>[12x]TKDNLTGDIVIIGAGAAGSLLAHYLARFSNMKIILLEAGHSHFNDPVVTDPMGFFGKYNPPNENISMSQNPSYSWQGAQEPNTGAYGNRPIIAHGMGFGGSTMINRLNLVVGGRTVFDNDWPVGWKYDDVKNYFRRVLVDINPVRDNTKASITSVALDALRIIAEQQIASGEPVDFLLNKATGNVPNVEKTTPDAVPLNLNDYEGVNSVVAFSSFYMGVNQLSDGNYIRKYAGNTYLNRNYVDENGRGIGKFSGLRVVSDAVVDRIIFKGNRAVGVNYIDREGIMHYVKVNKEVVVTSGAFYTPTILQRSGIGDFTYLSSIGVKNLVYNNPLVGTGLKNHYSPVTITRVHGEPSEVSRFLSNMAANPTNMGFKGLAELGFHRLDPNKPANANTVTYRKYQLMMTAGVGIPAEQQYLSGLSPSS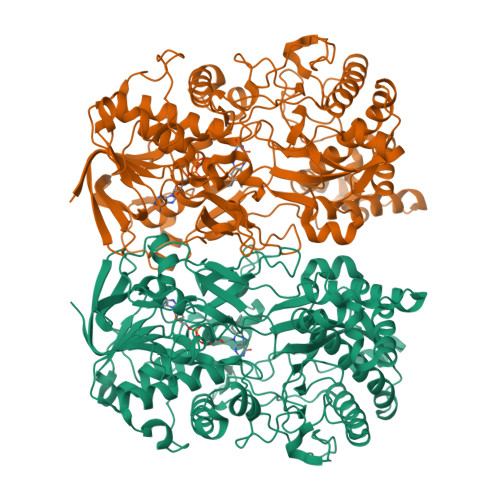NNLFTLIADDIRFAPEGYIKIGTPNIPRDVPKIFFNTFVTYTPTSAPADQQWPIAQKTLAPLISALLGYDIIYQTLMSMNQTARDSGFQVSLEMVYPLNDLIYKLHNGLATYGANWWHYFVPTLVGDDTPAGREFADTLSKLSYYPRVGAHLDSHQGCSCSIGRTVDSNLKVIGTQNVRVADLSAAAFPPGGNTWATASMIGARAVDLILGFPYLRDLPVNDVPILNVN>GSSDKGKLSLQDVAELIRARACQRVVVMVGAGISTPSGIPDFRSPGSGLYSNLQQYDLPYPEAIFELPFFFHNPKPFFTLAKELYPGNYKPNVTHYFLRLLHDKGLLLRL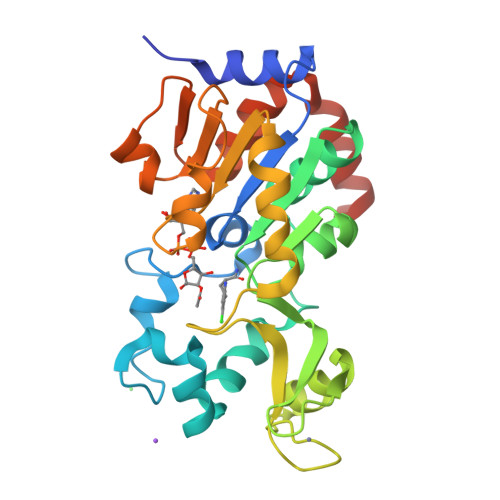YTQNIDGLERVSGIPASKLVEAHGTFASATCTVCQRPFPGEDIRADVMADRVPRCPVCTGVVKPDIVFFGEPLPQRFLLHVVDFPMADLLLILGTSLEVEPFASLTEAVRSSVPRLLINRDLVGPLAWHPRSRDVAQLGDVVHGVESLVELLGWTEEMRDLVQRETGKLDGPDK[3x]>[2x]MRGSHHHHHHGSSHANINAFKEAVTKIDRVEINRRLELAYAYNASIAGAKTNGEYPALIPNTGAEQKQAGVVEYARMLEV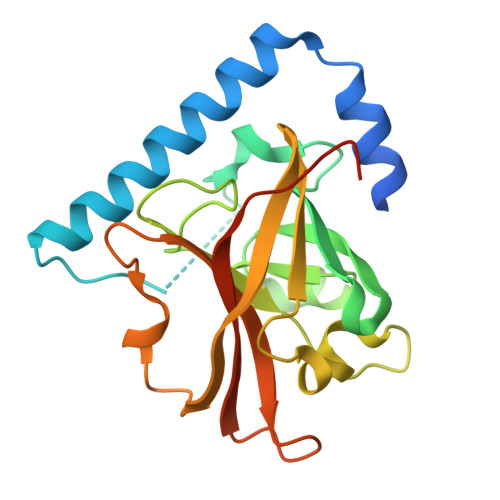KEQIGHVIIPRINQDIPIYAGSAEENLQRGVGHLEGTSLPVGGESTHAVLTAHRGLPTAKLFTNLDKVTVGDRFYIEHIGGKIAYQVDQIKVIAPDQLEDLYVIQGEDHVTLLTATPYMINSHRLLVRGKRIPYVEKTVQKDSKTFRQQQ>MGMKKSAVLNEHISKAIATIGHFDLLTINDAGMPIPNDHRRIDLAVTKNLPRFIDVLATVLEEMEIQK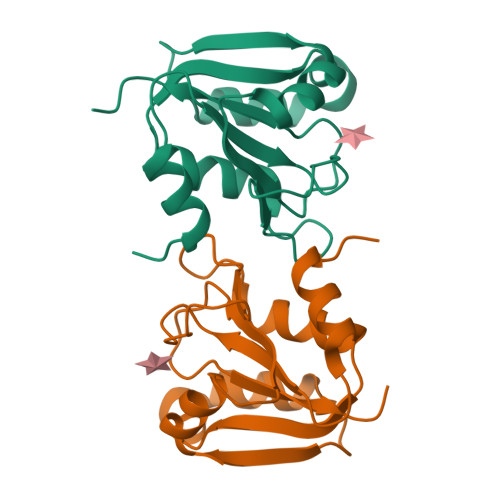IYLAEEIKEHNPTQLQQIKQLISSEIEIIFIPHEEMKSNLAHPLNKGNIRTGETTPYSNIALESNVTFLEHHHHHH[4x]>[3x]MHH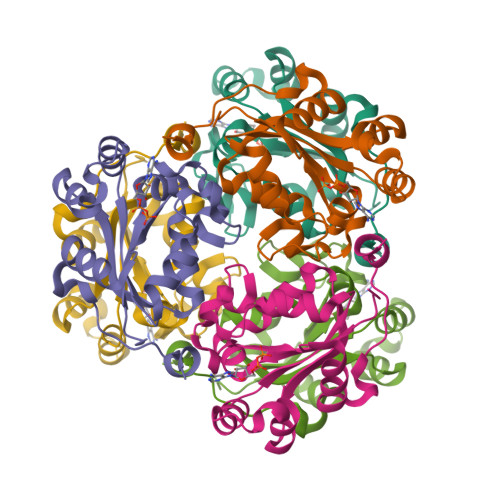HHHHGSMSNEQTFIAIKPDGVQRGLIGPIISRFENRGFKLVAMKLVSPPQSQLEQHYADLSDKPFFKGLVSYMLSGPICAMVWEGRDVVKTGRTILGATNPLASAPGTIRGDFAIDVGRNVCHGSDSVENAKKEIALWFKPEELISWKSATFDWVYEKA> KGHLTRLGLEFFDQPAVPLARAFLGQVLVRRLPNGTELRGRIVETEAYLGPEDEAAHSRGGRQTPRNRGMFMKPGTLYVYIIYGMYFCMNISSQGDGACVLLRALEPLEGLETMRHVRS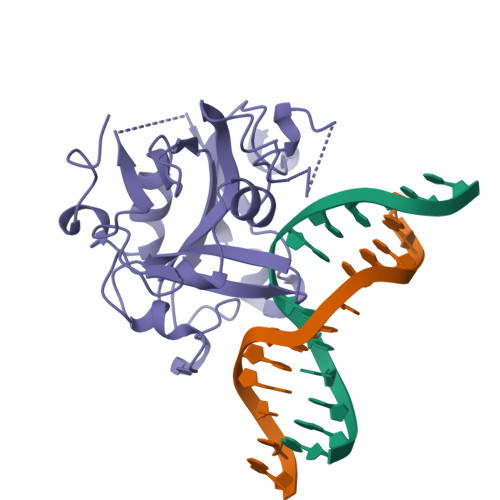QLRKGTASRVLKDRELCSGPSKLCQALAINKSFDQRDLAQDEAVWLERGPLEPSEPAVVAAARVGVGHAGEWARKPLRFYVRGSPWVSVVDRVAEQD>[2x]GMERAMEQLNRLTRSLRRARTVELPEDNETAVYTLMPMVMADQHRSVSELLSNSKFDVNYAFGRVKRSLLHIAANCGSVECLVLLLK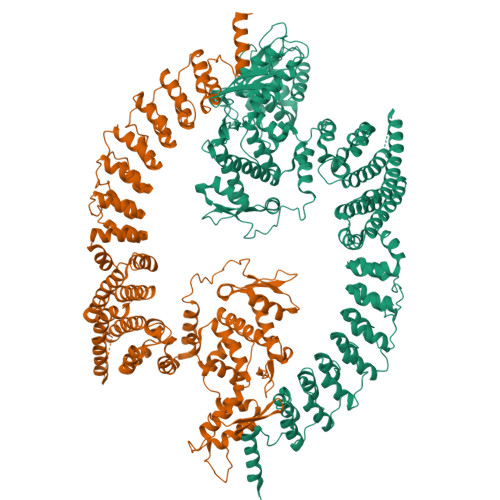KGANPNYQDISGCTPLHLAARNGQKKCMSKLLEYSADVNICNNEGLTAIHWLAVNGRTELLHDLVQHVSDVDVEDAMGQTALHVACQNGHKTTVQCLLDSGADINRPNVSGATPLYFACSHGQRDTAQILLLRGAKYLPDKNGVTPLDLCVQGGYGETCEVLIQYHPRLFQTIIQMTQNEDLRENMLRQVLEHLSQQSESQYLKILTSLAEVATTNGHKLLSLSSNYDAQMKSLLRIVRMFCHVFRIGPSSPSNGIDMGYNGNKTPRSQVFKPLELLWHSLDEWLVLIATELMKNKRDSTEITSILLKQKGQDQDAASIPPFEPPGPGSYENLSTGTRESKPDALAGRQEASADCQDVISMTANRLSAVIQAFYMCCSCQMPPGMTSPRFIEFVCKHDEVLKCFVNRNPKIIFDHFHFLLECPELMSRFMHIIKAQPFKDRCEWFYEHLHSGQPDSDMVHRPVNENDILLVHRDSIFRSSCEVVSKANCAKLKQGIAVRFHGEEGMGQGVVREWFDILSNEIVNPDYALFTQSADGTTFQPNSNSYVNPDHLNYFRFAGQILGLALNHRQLVNIYFTRSFYKHILGIPVNYQDVASIDPEYAKNLQWILDNDISDLGLELTFSVETDVFGAMEEVPLKPGGGSILVTQNNKAEYVQLVTELRMTRAIQPQINAFLQGFHMFIPPSLIQLFDEYELELLLSGMPEIDVSDWIKNTEYTSGYEREDPVIQWFWEVVEDITQEERVLLLQFVTGSSRVPHGGFANIMGGSGLQNFTIAAVPYTPNLLPTSSTCINMLKLPEYPSKEILKDRLLVALHCGSYGYTMA Here we used a functional analysis approach, coupled to detailed biochemistry and structural biology, to reveal a pathway for the degradation of plant N-glycans encoded by the human gut microbiota. We describe the biochemical characterization of five CAZymes and two crystal structures to provide a degradation pathway for plant complex N-glycans encoded by the human gut microbiome. In this study we characterize the likely pathway for the degradation of plant N-glycans by a prominent member of the human gut microbiota. B035DRAFT_03340GH92 is then able to remove the α1,3-mannose, followed by B035DRAFT_00995GH3 to cleave the plant-specific β1,2-xylose, and B035DRAFT_02132GH29 to release the core α1,3-fucose, leaving a Manα1,6Manβ1,4GlcNacβ1,4GlcNac tetrasaccharide.

To investigate the structural basis for specificity in the Bacteroides PNGase enzymes from group 2, we solved the crystal structure for B035DRAFT_03341PNGase to 1.95 Å. The structure consists of two domains: the catalytic domain and an NBL domain, which are linked through a flexible α-helical linker. The catalytic domain consists of two eight-stranded anti-parallel β-sheets, which is a consistent structural feature of PNGase enzymes described so far. The active site residues that are key for activity in EMTypeII are conserved in B035DRAFT_03341PNGase, with G388 occupying a critical position to allow the accommodation of α1,3-fucose. The available space for this fucose is particularly apparent in comparison to PNGaseF/EMTypeI. In contrast, the α1,6-fucose points away from the active site, so is not an issue in terms of blocking activity, consistent with the biochemical data. The NBL domain in the B. massiliensis structure has a very similar fold to the one in EMTypeII and is unique to these two proteins. They consist of 11 β-sheets connected by short α-helical regions and disordered loops. In contrast, the B. massiliensis PNGase from group 2 (B035DRAFT_03341PNGase) showed good activity toward plant-type N-glycans on HRP, with negligible activity against other structures. Overall these data show that B035DRAFT_03341PNGase requires a core α1,3-fucose for optimal activity (i.e., plant N-glycans), but that the presence of an α1,6-fucose can be accommodated (activity against insect N-glycans).

>MAAAAQNLQKKVKNAKGIEVIYQSSYKGKIRPGQIKMTVSGNQVALESVSPKGEKETATEGIREDKQPVIKNYIDYAGREAYKWAELPDGKIISAATPFEFGKGFTPAGEGKHLGLNCKIARTSINSNTIEVWYTHDIPFRGTPQANVGVPDGLVLKVVRNGDMIQEASAITPLKKAQALLPDSWGEKMDAADYQYTINQSGVITIPVFDQQTICFNNAKLPDTLEDGITYSAGGGTLILKKVKLPESAKNRSIFVEVAQYSDGDAYDRTGSVFVIPTDKKQSFLDAIRNLKSVPSFQAKDGNYPALISTDDYEAPVELMRFFTGFGVRKFNHNKVKGQHWVDSVIYKSEVTPLASQLQGEVWIGAYIGNWDAKGHRLSLKLKYYPDDERRVNKAMPLFNTVNYLEQAGQAYPVFFLNDSLRVRFTLKEPAKNARLFYLTTGHGGWGNGDEFNQKPNTVYLDGKKVISFIPWRDDCGTYRNSNPCSGNFSNGLSSSDLSRSNWCPGTVTTPEYIYLGDLEAGEHTLSVRIPQGAPEGGSNSYWCISGTLLYLEHHHHHH[2x]>[2x]MGSSHHHHHHSSGLVPRGSHMMHHHHHHHHGGVNQDFKVYLRLISYLKPYWGVALLVLIGFGMNSATEVSVAKLIKFIIDAIQNASRADLDWFPLLIILLVFFRGLGLFMGGYYTAVISRSLVFSIRQEVYAKLLRLPAQYYLDNSSGHITAKIMYNVEQLTAASSESLKTIVRDGMITLGLLGYLFYTNWRLTICIMVFLPIIGILVRKASKRMRKLSMQVQ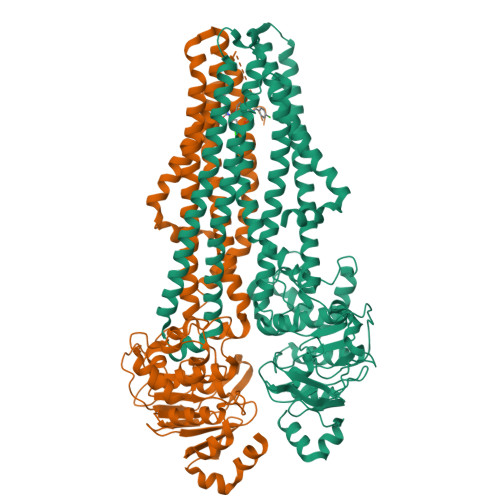DTMGDVNHVVQESINGNAVVKSFAGEESEQERFYKSSEENLKRGLKMVIVQNLNSPVVQVVMACAMALIVWLALRPQILGNTTAGEFVAYITAAGLLSKPVKNLTDVNEKLQRGLAAAHSVFELLDLPEEQNSGELKPQLQGAIRFDHVVLNYADGTQAIKDFSLDIRPGETVALVGRSGAGKTSLVNMLVRFQEVSSGQIYLDDLPIRDIELSSLRTQIAMVNQQVVLFNRTVRENIAYGQLHNASDEDVIAAAKAAYAHDFIMNLPNGYDTVLGAQGLNLSGGQRQRIAIARAILKNAPILILDEATSALDNESEHFIQQAFDEAMQDRTTIVIAHRLSTIENADRIVVMDRGQIVEQGTHQELLAKHGAYYQLHQRNFEDH In general, CIS are composed of a contractile sheath that surrounds an inner tube loaded with effectors, fitted with a baseplate complex. A conformational change in the baseplate complex triggers the contraction of the outer sheath, which leads to the propulsion of the inner tube into the target. Here we provide evidence that CIS from the model organism Streptomyces coelicolor (CISSc) function intracellularly and belong to a new class of CIS that exist as free-floating fully assembled particles in the cytoplasm and mediate cell death in response to stress conditions. Similar to the recently described sheath structures observed in AlgoCIS15 and tCIS19, the CISSc sheath is composed of a single protein, Cis2.

To obtain insights into the structural details of the CISSc contractile sheath-tube module, we performed single-particle cryoEM (helical reconstruction) of purified sheath particles from WT S. coelicolor, which had a homogeneous length for the contracted sheath of ~140 nm. The resulting map reached a resolution of 3.6 Å. Contracted sheath proteins adopt a right-handed helical array with an inner diameter of 115 Å and an outer diameter of 233 Å. Cis2 monomers consist of three domains and are well conserved in S. coelicolor and S. venezuelae, sharing ~65% sequence identity. From the resulting map, it was possible to build de novo domains 1 and 2, which contribute to the sheath wall. The additional domain 3, which is located on the sheath surface, seems to be highly flexible and could not be resolved. The overall contracted structure of Cis2 is similar to sheaths of previously characterized systems.

>MPSYLSPGVYVEEVASGSRPIEGVGTSVAAFVGLAPTGPLNEPTLVTNWTQYVAAFGDFTGGYYLAHSVYGFFNNGGSAAYVVRVGGSAEDAAADGSVNGAAAPAAVTGSTAKALPAAEPKQLGTFAVTATAAGQSGPLTVEVADPEGEGPAERFKLIVKDGDKPVETFDVSAKKGNRSYVVTQVKERSKLITVTEAAPSAQLVRPENQSLTLPAPPSAAPAVPAGQAESAHPGPAQYLGDSSDRTGFGGLEAIDEISMVAVPDLMAAYQRGAIDLEAVKAVQLGLIAHCELMGDRVAIIDPPPNQNARQIRVWRQETAGYDSKYAALYYPWIKSFDPATGQSRLVPPSGHVAGIWARNDSERGVHKAPANEVVRGAVDLELQITRGEQDLLNPIGVNCIRSFPGRGIRVWGARTLSSDPAWRYLNIRRYFNYLEESILIGTQWVVFEPNDHNLWARIRRNVSAFLVNEWRNGALFGQSPDQAYYVKCDEETNPPESVDLGRVVCEIGIAPVKPAEFVIFRLAQFSSGGGELDE[24x]The best characterized MoxR representative, the RavA protein, has been recently associated to oxidative stress, antibiotic resistance and iron-sulfur cluster assembly in Escherichia coli. Furthermore, it is involved in acid stress and nutrient stress responses via its interaction with the acid stress-inducible lysine decarboxylase LdcI, which buffers the bacterial cytoplasm by transforming lysine into cadaverine while consuming intracellular protons and producing CO2. Indeed, RavA is a 300 kDa lily-shaped hexameric ring, whereas LdcI is a 800 kDa toroid composed of two pentameric rings stacked together back-to-back. Here we present an 11 Å resolution cryo-electron microscopy (cryoEM) map of the LdcI–RavA complex and a 7.5 Å resolution cryoEM map of the LdcI-LARA complex, which together enable unambiguous flexible docking of the crystal structures, finally fitting together the pieces of the jigsaw.

We biochemically showed that the foot of RavA, inserted into the discontinuous triple helical bundle protruding as a leg from the AAA+ ATPase core, is necessary and sufficient for LdcI binding, albeit with a three orders of magnitude lower affinity. We therefore called this foot domain LARA for ‘LdcI associating domain of RavA’. As a result of these intricate rotations, both feet appear to interact with the inner or the outer rings of LdcI in exactly the same way. At this resolution, the crystal structures of LdcI and LARA can be docked into the EM density unambiguously because the secondary structure elements are clearly resolved. The LdcI decamer can be considered as barely affected by the LARA domain binding and all LdcI-LARA interaction sites are indeed equivalent. Noteworthy, it is the loop 329–360 of RavA which is responsible for the LdcI-LARA interaction.Video 3. Thus, critical residues in LdcI required for RavA binding were found to be E634 and Y697, both part of a C-terminal β-sheet. The charged residues R347 and R348 and the hydrophobic residues I343 and F344 at the tip of the LARA domain loop are required for RavA binding to LdcI. Thus, contrary to our earlier prediction based on the low resolution negative stain EM map, the LARA domain does not appear to directly block the access of ppGpp to its binding pocket but rather to induce a local conformational change in this pocket reducing ppGpp affinity.

> MNVIAILNHMGVYFKEEPIRELHRALERLNFQIVYPNDRDDLLKLIENNARLCGVIFDWDKYNLELCEEISKMNENLPLYAFANTYSTLDVSLNDLRLQISFFEYALGAAEDIANKIKQTTDEYINTILPPLTKALFKYVREGKYTFCTPGHMGGTAFQKSPVGSLFYDFFGPNTMKSDISISVSELGSLLDHSGPHKEAEQYIARVFNADRSYMVTNGTSTANKIVGMYSAPAGSTILIDRNCHKSLTHLMMMSDVTPIYFRPTRNAYGILGGIPQSEFQHATIAKRVKETPNATWPVHAVITNSTYDGLLYNTDFIKKTLDVKSIHFDSAWVPYTNFSPIYEGKCGMSGGRVEGKVIYETQSTHKLLAAFSQASMIHVKGDVNEETFNEAYMMHTTTSPHYGIVASTETAAAMMKGNAGKRLINGSIERAIKFRKEIKRLRTESDGWFFDVWQPDHIDTTECWPLRSDSTWHGFKNIDNEHMYLDPIKVTLLTPGMEKDGTMSDFGIPASIVAKYLDEHGIVVEKTGPYNLLFLFSIGIDKTKALSLLRALTDFKRAFDLNLRVKNMLPSLYREDPEFYENMRIQELAQNIHKLIVHHNLPDLMYRAFEVLPTMVMTPYAAFQKELHGMTEEVYLDEMVGRINANMILPYPPGVPLVMPGEMITEESRPVLEFLQMLCEIGAHYPGFETDIHGAYRQADGRYTVKVLKEESKK;> GHMQQSDKTALTVIRLGGIFSRRQQYQLPVNVTASTLTLLLQKPLKLHDMEVVHISFERSALEQWLSKGGEIRGKLNGIGFAQKLNLEVDSAQHLVVRDVSLQGSTLALPGSSAE>[2x]A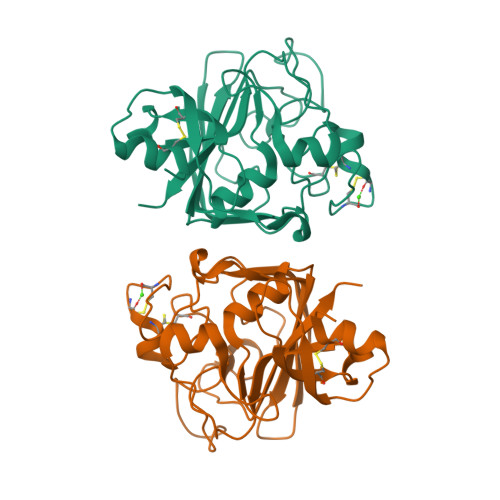DPFRDCADVYQAGFNKSGIYTIYINNMPEPKKVFCNMDVNGGGWTVIQHREDGSLDFQRGWKEYKMGFGNPSGEYWLGNEFIFAITSQRQYMLRIELMDWEGNRAYSQYDRFHIGNEKQNYRLYLKGHTGTAGKQSSLILHGADFSTKDADNDNCMCKCALMLTGGWWFDACGPSNLNGMFYTAGQNHGKLNGIKWHYFKGPSYSLRSTTMMIRPLDGGR>[2x]MFAGLQDLGVANGEDLKETLTNCTEPLKAIEQFQTENGVLLPSLQSALPFLDLHGTPRLEFHQSVFDELRDKLLERVSAIASEGKAEERYKKLEDLLE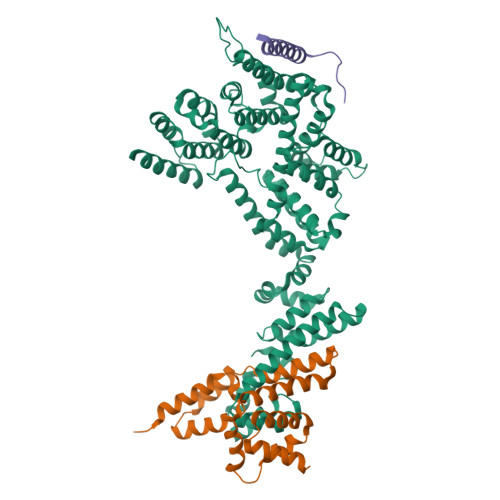KSFSLVKMPSLQPVVMCVMKHLPKVPEKKLKLVMADKELYRACAVEVKRQIWQDNQALFGDEVSPLLKQYILEKESALFSTELSVLHNFFSPSPKTRRQGEVVQRLTRMVGKNVKLYDMVLQFLRTLFLRTRNVHYCTLRAELLMSLHDLDVGEICTVDPCHKFTWCLDACIRERFVDSKRARELQGFLDGVKKGQEQVLGDLSMILCDPFAINTLALSTVRHLQELVGQETLPRDSPDLLLLLRLLALGQGAWDMIDSQVFKEPKMEVELITRFLPMLMSFLVDDYTFNVDQKLPAEEKAPVSYPNTLPESFTKFLQEQRMACEVGLYYVLHITKQRNKNALLRLLPGLVETFGDLAFGDIFLHLLTGNLALLADEFALEDFCSSLFDGFFLTASPRKENVHRHALRLLIHLHPRVAPSKLEALQKALEPTGQSGEAVKELYSQLGEKLEQLDHRKPSPAQ;>EGEDDAEVQQECLHKFSTRDYIMEPSIFNTLKRYFQAGGSPENVIQLLSENYTAVAQTVNLLAEWLIQTGVEPVQVQETVENHLKSLLIKHFDPRKADSIFTEEGETPAWLEQMIAHTTWRDLFYKLAEAHPDCLMLNFTVKLISDA[2x];>[2x]MLVIPPGMSEEEEALQKKFMKLKKKKKALMALKKQSSSSTTSQGGVKRSLY> MQTEHVILLNAQGVPTGTLEKYAAHTADTRLHLAFSSW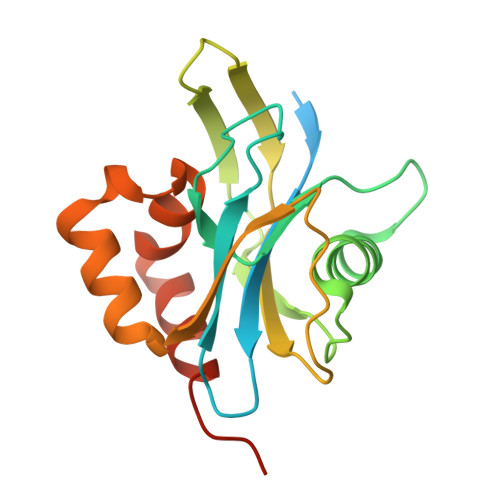LFNAKGQLLVTRRALSKKAWPGVWTNSVCGHPQLGESNEDAVIRRCRYELGVEITPPESIYPDFRYRATDPSGIVENEVCPVFAARTTSALQINDDEVMDYQWCDLADVLHGIDATPWAFSPWMVMQATNREARKRLSAFTQLKLEHHHHHH>[5x]MGNDISLIALLAFSTLLPFIIASGTCFVKFSIVFVMVRNALGLQQIPSNMTLNGVALLLSMFVMWPIMHDAYVYFEDEDVTFNDISSLSKHVDEGLDGYRDYLIKYSDRELVQFFENAQLKRQYGEETETVKRDKDEIEKPSIFALLPAYALSEIKSAFKIGFYLYLPFVVVDLVVSSVLLALGMMMMSPVTISTPIKLVLFVALDGWTLLSKGLILQYMDIAT;> MFYALYFEIHHLVASAALGFARVAPIFFFLPFLNSGVLSGAPRNAIIILVALGVWPHALNEAPPFLSVAMIPLVLQEAAVGVMLGCLLSWPFWVMHALGCIIDNQRGATLSSSIDPANGIDTSEMANFLNMFAAVVYLQ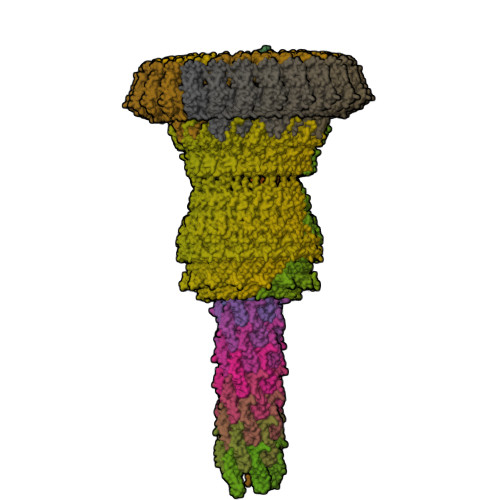NGGLVTMVDVLNKSYQLCDPMNECTPSLPPLLTFINQVAQNALVLASPVVLVLLLSEVFLGLLSRFAPQMNAFAISLTVKSGIAVLIMLLYFSPVLPDNVLRLSFQATGLSSWFYERGATHVLE;>MDDLVFAGNKALYLVLILSGWPTIVATIIGLLVGLFQTVTQLQEQTLPFGIKLLGVCLCLFLLSGWYGEVLLSYGRQVIFLALAKG[4x];>MSIATIVPENAVIGQAVNIRSMETDIVSLDDRLLQAFSGSAIATAVDKQTITNRIEDPNLVTDPKELAISQEMISDYNLYVSMVSTLTRKGVGAVETLLRS[6x];>[72x]MATPWSGYLDDVSAKFDTGVDNLQTQVTEALDKLAAKPSDPALLAAYQSKLSEYNLYRNAQSNTVKVFKDIDAAIIQNFR;>[16x]MKTHILLARVLACAALVLVTPGYSSEKIPVTGSGFVAKDDSLRTFFDAMALQLKEPVIVSKMAARKKITGNFEFHDPNALLEKLSLQLGLIWYFDGQAIYIYDASEMRNAVVSLRNVSLNEFNNFLKRSGLYNKNYPLRGDNRKGTFYVSGPPVYVDMVVNAATMMDKQNDGIELGRQKIGVMRLNNTFVGDRTYNLRDQKMVIPGIATAIERLLQGEEQPLGNIVSSEPPAMPAFSANGEKGKAANYAGGMSLQEALKQNAAAGNIKIVAYPDTNSLLVKGTAEQVHFIEMLVKALDVAKRHVELSLWIVDLNKSDLERLGTSWSGSITIGDKLGVSLNQSSISTLDGSRFIAAVNALEEKKQATVVSRPVLLTQENVPAIFDNNRTFYTKLIGERNVALEHVTYGTMIRVLPRFSADGQIEMSLDIEDGNDKTPQSDTTTSVDALPEVGRTLISTIARVPHGKSLLVGGYTRDANTDTVQSIPFLGKLPLIGSLFRYSSKNKSNVVRVFMIEPKEIVDPLTPDASESVNNILKQSGAWSGDDKLQKWVRVYLDRGQEAIK;>[24x]MIRRYLYTFLLVMTLAGCKDKDLLKGLDQEQANEVIAVLQMHNIEANKIDSGKLGYSITVAEPDFTAAVYWIKTYQLPPRPRVEIAQMFPADSLVSSPRAEKARLYSAIEQRLEQSLQTMEGVLSARVHISYDIDAGENGRPPKPVHLSALAVYERGSPLAHQISDIKRFLKNSFADVDYDNISVVLSERSDAQLQAPGTPVKRNSFATSWIVLIILLSVMSAGFGVWYYKNHYARNKKGITADDKAKSSNE;>METSKEKTITSPGPYIVRLLNSSLNGCEFPLLTGRTLFVVGQSDALTASGQLPDIPADSFFIPLDHGGVNFEIQVDTDATEIILHELKEGNSESRSVQLNTPIQVGELLILIRPESEPWVPEQPEKLETSAKKNEPRFKNGIVAALAGFFILGIGTVGTLWILNSPQRQAAELDSLLGQEKERFQVLPGRDKMLYVAAQNERDTLWARQVLARGDYDKNARVINENEENKRISIWLDTYYPQLAYYRIHFDEPRKPVFWLSRQRNTMSKKELEVLSQKLRALMPYADSVNITLMDDVTAAGQAEAGLKQQALPYSRRNHKGGVTFVIQGALDDVEILRARQFVDSYYRTWGGRYVQFAIELKDDWLKGRSFQYGAEGYIKMSPGHWYFPSPL[24x]>GSMTGKSVKDVDRYQAVLANLLLEEDNKFCADCQSKGPRWASWNIGVFICIRCAG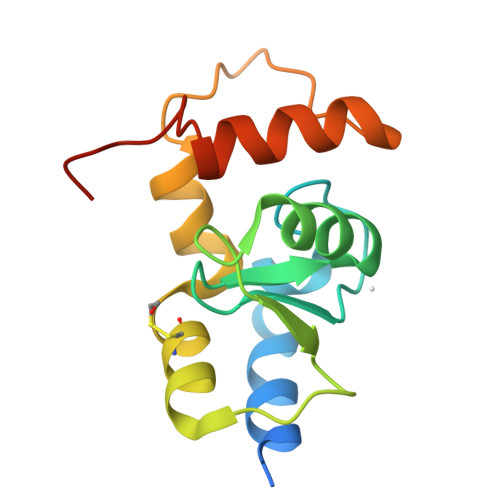IHRNLGVHISRVKSVNLDQWTQEQIQCMQEMGNGKANRLYEAYLPETFRRPQIDPAVEGFIRDKYEKKKYMDRSLDINA[2x]In this study, we report the crystal structure of CsgC, the first among the Csg proteins to be solved. The overall structure of CsgC consists of an immunoglobulin (Ig)-like β sandwich with seven strands forming two sheets and well-defined loop regions. The protein adopts an immunoglobulin-like fold and contains an unusual invariant CxC motif reminiscent of the oxido-reductase superfamily CxxC motif. Based on its similarity to the N-terminal domain of DsbD, we propose that CsgC has redox activity and CsgG is the potential substrate.

We obtained structures of CsgC in which the cysteines were either oxidized or reduced. There were no gross structural changes associated with disulfide bond formation (root-mean-square deviation [rmsd] Cα backbone atoms = 0.65 Å), which is consistent with the high degree of similarity observed between NMR spectra of reduced and oxidized CsgC. In order to confirm the oxidation state of CsgC in vitro, mass spectrometry was used to measure accurate molecular weights for the oxidized and reduced forms. The reduced protein had a molecular weight of 12,066 Da, however after incubation with oxidized glutathione (GSSG) this decreased by 2 Da, indicating formation of the disulfide. Strikingly, the introduction of the disulfide bond caused a large increase in protein stability, as evidenced by a shift in the thermal melting midpoint Tm value from 66.1 ± 0.5°C to 92.4 ± 0.8°C. A unique feature of the CsgC structure is the invariant CxC motif that connects the BC loop to strand C. Similarly, the CxC motif of CsgC is partially buried and the intervening side chain is always an exposed, nonpolar residue (L/V). The cysteine residues are located in the “complementarity-determining region” (CDR) of the Ig fold, a common site of target recognition, suggesting that they could be key to the cellular function of CsgC.

> MGSSQITFNTTQQGDMYTIIPEVTLTQSCLCRVQILSLREGSSGQSQTKQEKTLSLPANQPIALTKLSLNISPDDRVKIVVTVSDGQSLHLSQQWPPSSEKSLEHHHHHH> MSKLDSLLKELPTRTAHLYRSIWHKYTEWLKTMPDLTGADLKLFLSQKYIVKYIASHDDIAKDPLPTCDAMIWFSRALDIENNDVLVLQQRLYGLVKLLEFDYSNVIAILQKISINLWNPSTDSLQSKHFKTCQDKLKLLLDFQWKFNTNVSFEDRTTVSLKDLQCILDDENGKCGLAHSSKPNFVLVPNFQSPFTCPIFTMAVYYYLRFHGVKKYYKGDGYQILSQLEHIPIIRGKSLDQYPRELTLGNWYPTIFKYCQLPYTKKHWFQVNQEWPQFPDFSD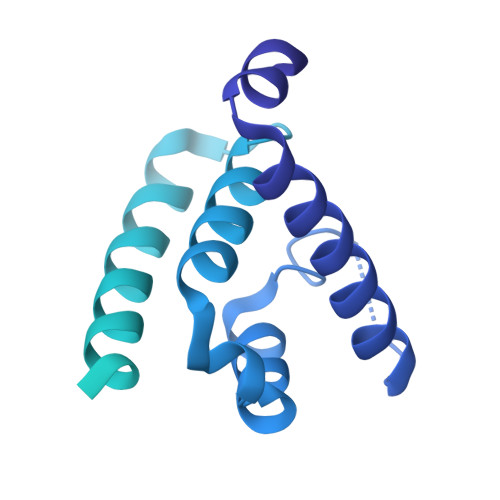SSENTSTLAESDSENTIGIPDFYIEKMNRTKLQPCPQVHVHLFPTDLPPDIQAVFDLLNSVLVTSLPLLYRVFPTHDIFLDPSLKTPQNIAFLTGTLPLDIESQEHLLAQLIDKTGTVSEIGSG> MLDRIASIKKAPDEEYYVPGH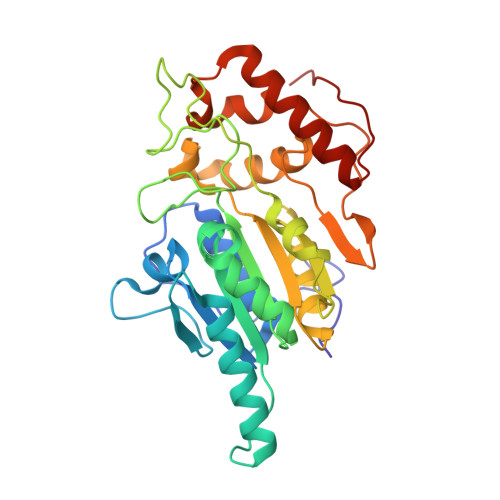RTCAGCGPALTYRLVAKAAGPNTIFIGPTGCMYVANTSYGCGPWRVPWIHAQITNGGAVASGIEAAYKAMIRKKKTDAEFPNIIVMAGDGGAVDIGLQALSAMLYRGHDVLFICYDNESYANTGIQTSPTTPYGANTTFTPPGEVVPEGKKLFPKDNPKVIAHGHPELKYVATASIGWPVDLMNKVRKGLNQEGPAYIHIHAPCPKGWQFPADKTIEMAKLAVQTGMFQLYEYENGEYKLSVKVDKRKPVSEYMKLQKRFAHLKPEHIAKMQAFVDARCAEVGITVPVVASNA>GSHMDPKLPETSSRQPVYHNLTIEENIINLKQKIYDNATKITNIDKGLQGSITDDQKENLLKLKENYKQLIDNQKEQLKTYK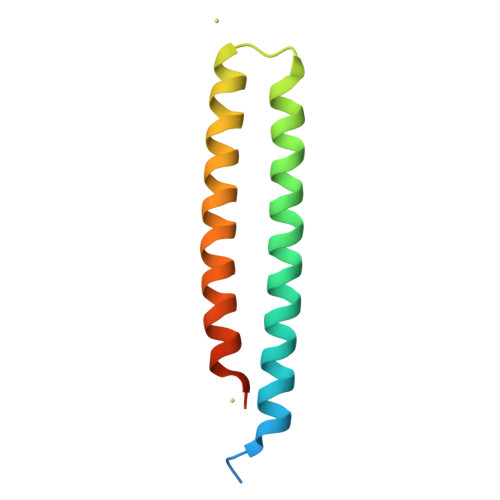NLLNDLNDEKN[2x]> MIDAESPTTAFRTKPAPVDPSLQHEIEQFYYWEAKLLNDRRFQEWFDLLAEDIHYFMPIRTTRIMRETAQEYSGAREYAHFDDNAQMMRGRLRKITSDVSWSENPASRTRHVISNVMIVDGEKPGE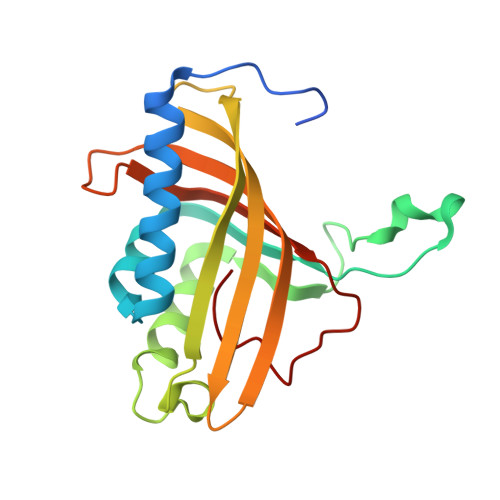YHVSSVFIVYRNRLERQLDIFAGERKDILRRTGSEAGFELAKRTILIDQSTILSNNLSFFF>MNTP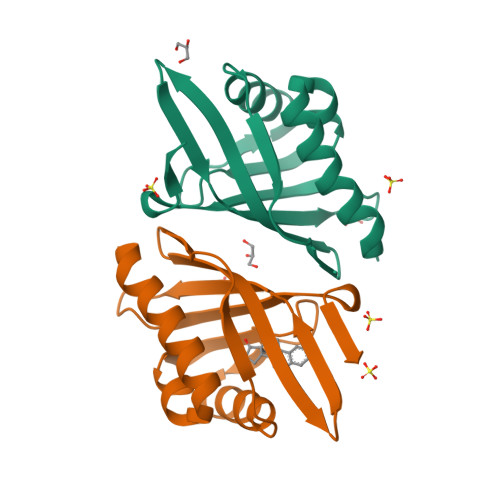EHMTAVVQRYVAALNAGDLDGIVALFADDATVEDPVGSEPRSGTAAIREFYANSLKLPLAVELTQEVRAVANEAAFAFTVSFEYQGRKTVVAPINHFRFNGAGKVVSMRALFGEKNIHAGA[4x]>[2x]AMAGVYTYENEFTSDIPAPKLFKAFVLDADNLIPKIAPQAVKCAEILEGDGGPGTIKKITFGEGSHYGYVKHKIHSIDKVNHTYSYSLIEGDALSENIEKIDYETKLVSAPHGGTIIKTTSKYHTKGDVEIKEEHVKAGKEKAAHLFKLIEGYLKDHPSEYN

Fra a proteins are members of the pathogenesis-related 10 family and are required for the normal accumulation of flavonoids and the development of color in strawberry fruits. PR-10 proteins belong to the START superfamily. These proteins adopt a helix-grip fold with an internal cavity capable of binding hydrophobic ligands. The data presented here demonstrates that Fra a proteins bind natural flavonoids, providing for the first time mechanistic insight on the function of these proteins in the control of flavonoid biosynthesis.

The Fra a 1E protein crystallized in two different crystal forms. The two crystal forms belong to the same space group (P212121) but show different unit cell dimensions and molecular arrangement. Crystal form A contains two protein molecules per asymmetric unit, whereas crystal from B contains six independent copies per asymmetric unit. The refined model contained two molecules of Fra a 1E in the asymmetric unit. Both molecules showed a similar structure and comprise amino acids 2 to 160. The region corresponding to the β3-β4 loop (amino acids 61–63 and 61–65 in chains A and B, respectively) was disordered and could not be modeled. The three amino acids from the N-terminal purification tag that remain after TEV cleavage were also visible in the structure. As can be appreciated in Fig. 3a, the structure of Fra a 1E conforms to the START fold and consists of a seven-stranded β-sheet, two short helical segments between strands 5 and 7, and a long α-helix at the C terminus. The β-sheet adopts a slightly curved shape with the long C-terminal α-helix (α3) juxtaposed against the concave side, which creates a cavity in the middle of the protein. The open end of the cavity was surrounded by loops α2-β2, β3-β4, β5-β6, and β7-α3, designated here, respectively, as L3 (amino acids 35–39), L5 (amino acids 60–65), L7 (amino acids 89–96), and L9 (amino acids 125–130), and by the N-terminal half of the last α-helix (α3). A number of well ordered water molecules were found inside the cavity.> GSAPYASLTEIEHLVQSVCKSYRETCQLRLEDLLRQRSNIFSRE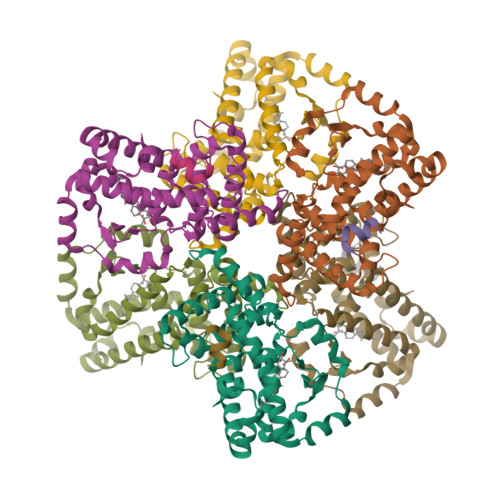EVTGYQRKSMWEMWERCAHHLTEAIQYVVEFAKRLSGFMELCQNDQIVLLKAGAMEVVLVRMCRAYNADNRTVFFEGKYGGMELFRALGCSELISSIFDFSHSLSALHFSEDEIALYTALVLINAHRPGLQEKRKVEQLQYNLELAFHHHLCKTHRQSILAKLPPKGKLRSLCSQHVERLQIFQHLHPIVVQAAFPPLYKELFSTETESPVGLSK;> TLLQLLLGHKNE>[2x]MSNTISEKIVLMRKSEYLSRQQLADLTGVPYGTLSYYESGRSTPPTD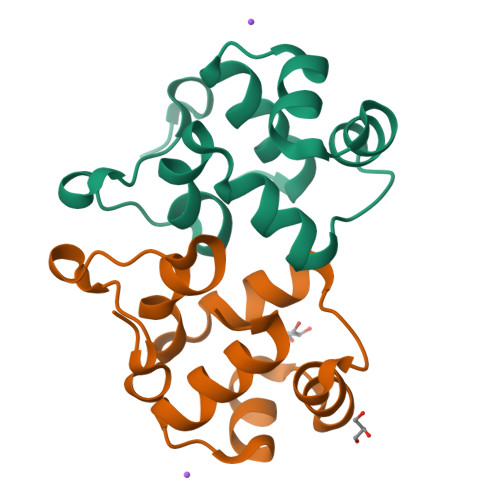VMMNILQTPQFTKYTLWFMTNQIAPESGQIAPALAHFGQNETTSPHSGQKTG>ATDGSHFDFVIVGGGTAGNTVAGRLAENPNVTVLIVEAGIGNPEDIPEITTPSSAMDLRNSKYDWAYKTTMVRRDDYERIEKPNTRGKTLGGSSSLNYFTWVPGHKATFDQWEEFGGKEWTWDPLVPYLRKSATYHDDPRLYSPELEKIGGGGPIPISHAELIDEMAPFRENLTKAWKSMGQPLIENIYDGEMDGLTHCCDTIYRGQRSGSFLFVKNKPNITIVPEVHSKRLIINEADRTCKGVTVVTAAGNELNFFADREVILSQGVFETPKLLMLSGIGPTRELSRHGINTIVDSRHVGQNLMDHPGVPFVLRVKDGFGMDDVLLRHGPKRDAVVSAYNKNRSGPVGSGLLELVGFPRIDKYLEKDAEYRKAKAANGGKDPFSPLGQPHFELDFVCMFGTAFQWHFPTPKTGDHLTVVVDLVRPISDPGEVTLNSADPFQQPNINLNFFANDLDIIAMREGIRFSYDLLFKGEGFKDLVESEYPWE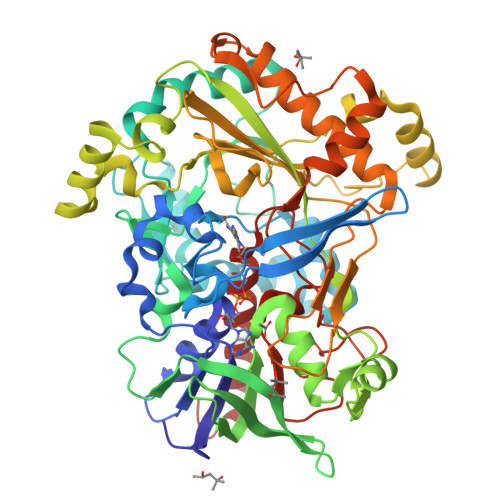MPLDSDKEMHRAVLDRCQTAFHPTGTARLSKNIDQGVVDPKLKVHGIKKLRVADASVIPIIPDCKIQNSVYAVGEKCADMIKAEHKDLY[3x]>[4x]MSFPGWGPYPPVERDETSAITYSSKLHGSVTVRDPYSQLEVPFEDSEETKAFVHSQRKFARTYLDENPDREAWLETLKKS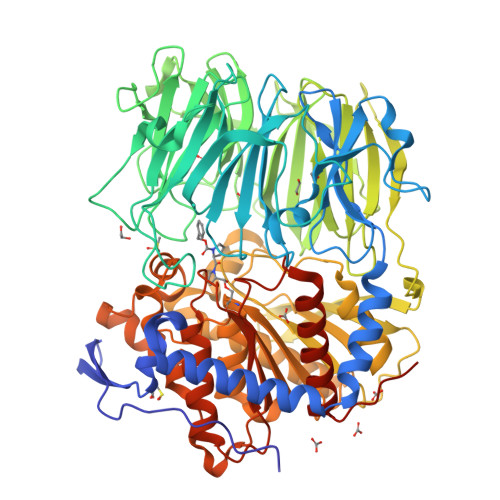WNYRRFSALKPESDGHYYFEYNDGLQSQLSLYRVRMGEEDTVLTESGPGGELFFNPNLLSLDGNAALTGFVMSPCGNYWAYGVSEHGSDWMSIYVRKTSSPHLPSQERGKDPGRMNDKIRHVRFFIVSWTSDSKGFFYSRYPPEDDEGKGNAPAMNCMVYYHRIGEDQESDVLVHEDPEHPFWISSVQLTPSGRYILFAASRDASHTQLVKIADLHENDIGTNMKWKNLHDPWEARFTIVGDEGSKIYFMTNLKAKNYKVATFDANHPDEGLTTLIAEDPNAFLVSASIHAQDKLLLVYLRNASHEIHIRDLTTGKPLGRIFEDLLGQFMVSGRRQDNDIFVLFSSFLSPGTVYRYTFGEEKGYRSLFRAISIPGLNLDDFMTESVFYPSKDGTSVHMFITRPKDVLLDGTSPVLQYGYGGFSLAMLPTFSLSTLLFCKIYRAIYAIPNIRGGSEYGESWHREGMLDKKQNVFDDFNAATEWLIANKYASKDRIAIRGGSNGGVLTTACANQAPGLYRCVITIEGIIDMLRFPKFTFGASWRSEYGDPEDPEDFDFIFKYSPYHNIPPPGDTVMPAMLFFTAAYDDRVSPLHTFKHVAALQHNFPKGPNPCLMRIDLNSGHFAGKSTQEMLEETADEYSFIGKSMGLTMQTQGSVDSSRWSCVTV>[2x]MQNPINDLRSAIALLQRHPGHYIETDHPVDPNAELAGVYR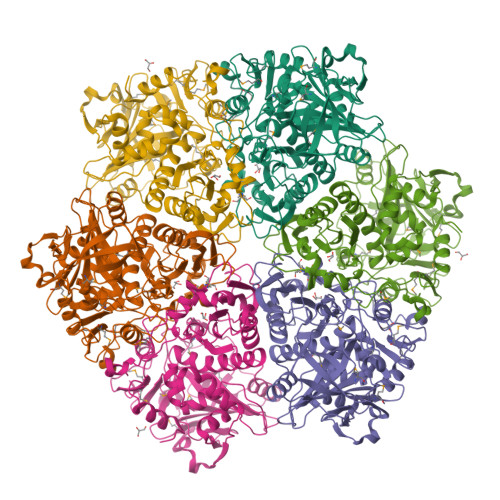HIGAGGTVKRPTRTGPAMMFNSVKGYPGSRILVGMHASRERAALLLGCVPSKLAQHVGQAVKNPVAPVVVPASQAPCQEQVFYADDPDFDLRKLLPAPTNTPIDAGPFFCLGLVLASDPEDTSLTDVTIHRLCVQERDELSMFLAAGRHIEVFRKKAEAAGKPLPVTINMGLDPAIYIGACFEAPTTPFGYNELGVAGALRQQPVELVQGVAVKEKAIARAEIIIEGELLPGVRVREDQHTNTGHAMPEFPGYCGEANPSLPVIKVKAVTMRNHAILQTLVGPGEEHTTLAGLPTEASIRNAVEEAIPGFLQNVYAHTAGGGKFLGILQVKKRQPSDEGRQGQAALIALATYSELKNIILVDEDVDIFDSDDILWAMTTRMQGDVSITTLPGIRGHQLDPSQSPDYSTSIRGNGISCKTIFDCTVPWALKARFERAPFMEVDPTPWAPELFSDKK> MSLAHTAAEYMLSDALLPDRRGPRLKGLRLELPLDRIVKFVAVGSPLLLMSLAFAQEFSSGSPISCFSPSNFSIRQAAYVDSSCWDSLLHHKQDGPGQDKMKSLWPHKALPYSLLALALLMYLPVLLWQYAAVPALSSDLLFIISELDKSYNRSIRLVQHMLKIRQKSSDPYVFWNELEKARKERYFEFPLLERYLACKQRSHSLVATYLLRNSLLLIFTSATYLYLGHFHLDVFFQEEFSCSIKTGLLSDETHVPNL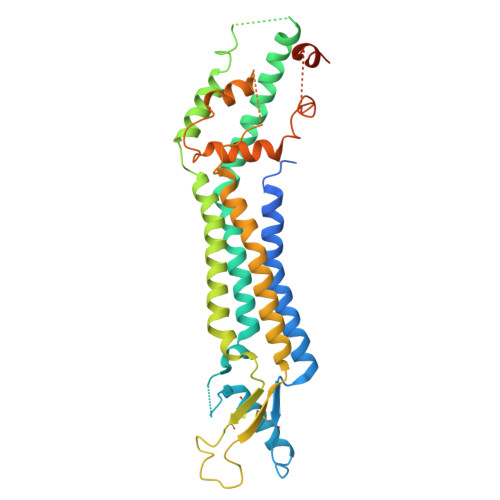ITCRLTSLSIFQIVSLSSVAIYTILVPVIIYNLTRLCRWDKRLLSVYEMLPAFDLLSRKMLGCPINDLNVILLFLRANISELISFSWLSVLCVLKDTTTQKHNIDTVVDFMTLLAGLEPSKPKHLTNSACDEHPGSGGSGHHHHHH>MKLYVFLVNTGTTLTFDTELTVQTVADLKHAIQSKYKIAIQHQVLVVNGGECMAADRRVCTYSAGTDTNPIFLFNKEMILCDRPPAIPKTTFSTENDMEIKVEESLMMPAVFHTVASRTQLALEMYEVAKKLCSFCEGLVHDEHLQHQGWAAIMANLEDCSNSYQKLLFKFESIYSNYLQSIEDIKLKLTHLGTAVSVMAKIPLLECLTRHSYRECLGRLDSLPEHEDSEKAEMKRSTELVLSPDMPRTTNESLLTSFPKSVEHVSPDTADAESGKEIRESCQSTVHQQDETTIDTKDGDLPFFNVSLLDWINVQDRPNDVESLVRKCFDSMSRLDPRIIRPFIAECRQTIAKLDNQNMKAIKGLEDRLYALDQMIASCGRLVNEQKELAQGFLANQKRAENLKDASVLPDLCLSHANQLMIMLQNHRKLLDIKQKCTTAKQELANNLHVRLKWCCFVMLHADQDGEKLQALLRLVIELLERVKIVEALSTVPQMYCLAVVEVVRRKMFIKHYREWAGALVKDGKRLYEAEKSKRESFGKLFRKSFLRNRLFRGLDSWPPSFCTQKPRKFDCELPDISLKDLQFLQSFCPSEVQPFLRVPLLCDFEPLHQHVLALHNLVKAAQSLDEMSQTITDLLSEQK[2x];>[2x]MEQEHTEILRGLRFTLLFVQHVLEIAALKGSASEAAGGPEYQLQESVVADQISLLSREWGFAEQLVLYLKVAELLSSGLQSAIDQIRAGKLCLSSTVKQVVRRLNELYKASVVSCQGLSLRLQRFFLDKQRLLDRIHSITAERLIFSHAVQMVQSAALDEMFQHREGCVPRYHKALLLLEGLQHMLSDQADIENVTKCKLCIERRLSALLTGICA;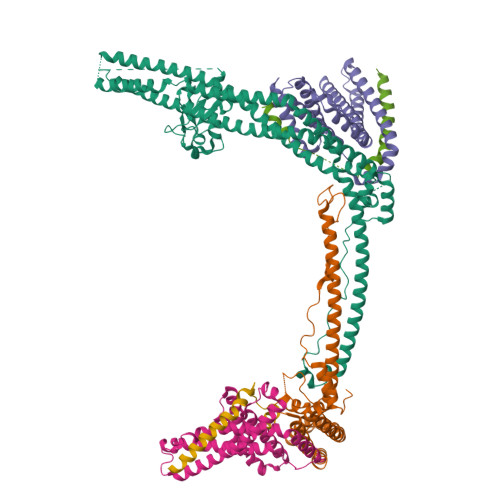>[2x]KPAFSKDDILPMDLGTFYREFQNPPQLSSLSIDIGAQSMAEDLDSLPEKLAVHEKNVREFDAFVETLQGSDEA4-amino-N-[(1S)-1-(4-chlorophenyl)-3-hydroxypropyl]-1-(7H-pyrrolo[2,3-d]pyrimidin-4-yl)piperidine-4-carboxamide 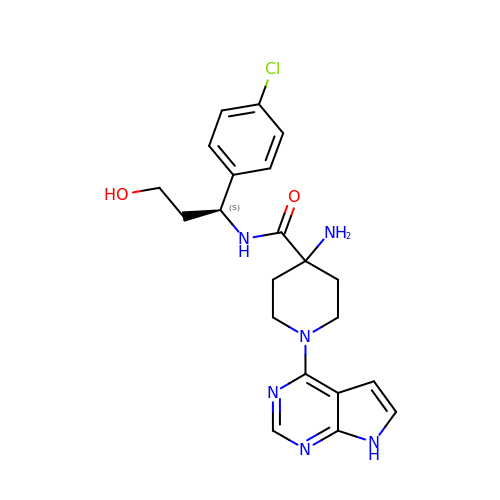| C21 H25 Cl N6 O2 | JDUBGYFRJFOXQC-KRWDZBQOSA-N>[2x]SGGGMLTLIQGKKIVNHLRSRLAFEYNGQLIKILSKNIVAVGSLR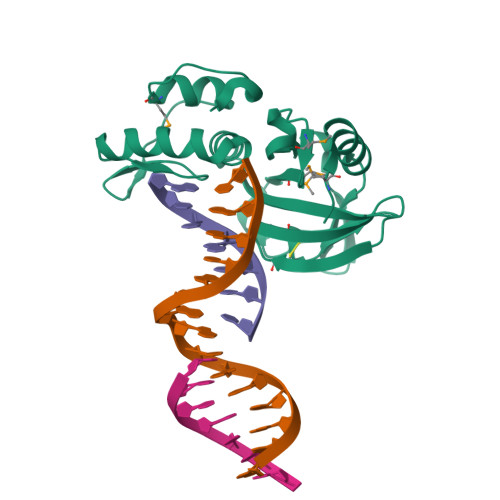REEKMLNDVDMLIIVPEKKLLKHVLPNIRIKGLSFSVKVCGERKCVLFIEWEKKTYQLDLFTALAEEKPYAIFHFTGPVSYLIRIRAALKKKNYKLNQYGLFKNQTLVPLKITTEKELIKEMGFTYRIPKKRL Expanding this pattern to hpphhph can produce larger α-helical barrels. Here, we show that pentameric to nonameric barrels are accessed by varying the residue at one of the h sites. In peptides with four L/I–K–E–I–A–x–Z repeats, decreasing the size of Z from threonine to serine to alanine to glycine gives progressively larger oligomers. X-ray crystal structures of the resulting α-helical barrels rationalize this: side chains at Z point directly into the helical interfaces, and smaller residues allow closer helix contacts and larger assemblies.

Conversely, both Gly variants scored more favourably as larger oligomeric states: the a = d = Ile variant as an octamer; and a = Leu, d = Ile as a nonamer. The Gly@g peptide with a = Leu, d = Ile crystallized in two forms. Gratifyingly, one was an all-parallel nonamer, which is a new αHB with an exceptionally large channel of diameter ≈9.5–11.5 Å, Fig. 3 (Table S4†). Attempts to model solvent into density observed in the channel were inconsistent. Therefore, representative solvent molecules were included where they matched the density; though these did not make any stabilizing contacts with protein. Although there are natural nonameric protein assemblies, this is the first stand-alone, water-soluble α-helical CC of this size. In addition, the crystallization conditions for the octamer and nonamer contained isopropanol. This increases the hydrophobicity of the bulk solvent, which potentially supports larger, hydrophobic pores that would otherwise be energetically unfavourable.

>[36x]XGEIAQGLKEIAKGLKEIAWGLKEIAQGLKGX> PETLVKVKDAEDQLCRTSHRPCRVGYIELDLNSGKILESFRPEERFPMMSTFKVLLCGAVLSRIDAGQEQLGRRIHYSQNDLVKYSPVTEKHLTDGMTVRELCSAAITMSDNTAANLLLTTIGGPKELTAFLHNMGDHVTRLDRWEPELNEAIPNDERDTTMPVAMATTLRKLLTGELLTLASRQQLIDWM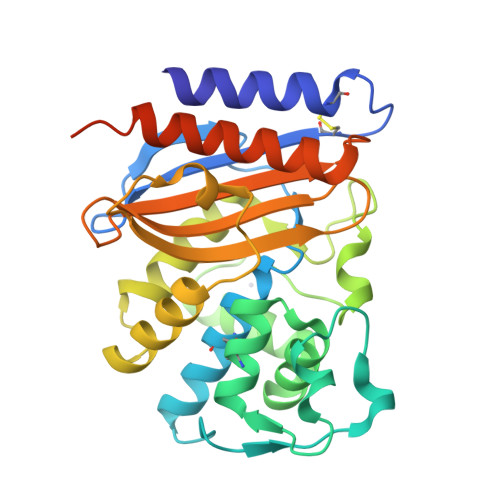EADKVAGPLLRSALPAGWFIADKSGAGRRGSRGIIAALGPDGKPSRIVVIYTTGSRKKTDERNRQIAEIGASLIKHWGLEQKLISEEDLNSAVDHHHHHH>MTNSNNRQSEYPVDPLFLDRWSPRAFDGSPMPKEHLLTILDAAHWAPSASNHQPWRFVYAHKDSEDWPLFVELLMEGNQKWAKNASVLLFVISRDHTISHEGEKKPSATHSFDAGAAWFSLAMQAHLLGYHAHGMGGIFKDRIVEKLDIPDGFKVEAGVAIGTLTDKSILP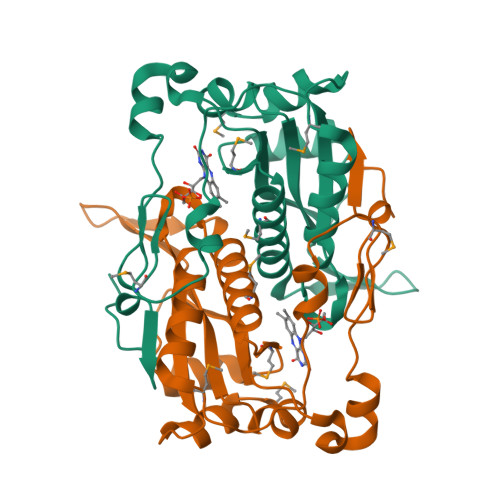DDLAEREVPSKRVPLADVAFEGRFTGKAD[2x]(5-chloro-1-benzothiophen-3-yl)acetic 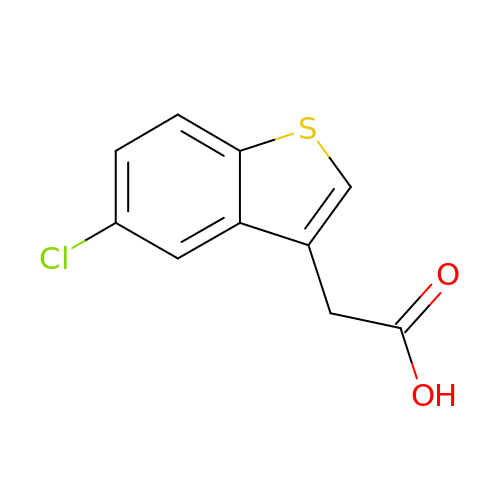acid | C10 H7 Cl O2 S | QQKKTOPRRGBBCT-UHFFFAOYSA-N(5Z)-5-(carbamoylimino)-3-[(5R)-6,7,8,9-tetrahydro-5H-benzo[7]annulen-5-ylsulfanyl]-2,5-dihydroisothiazole-4-carboxamide 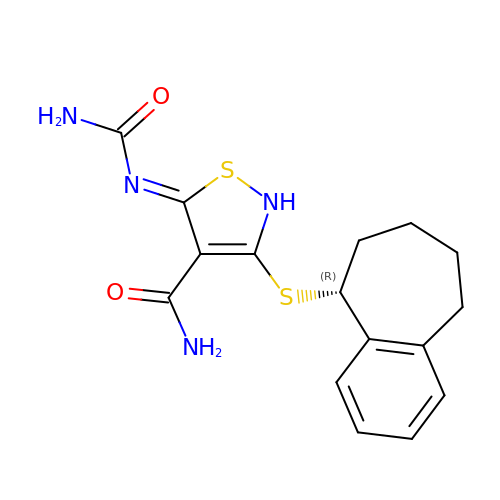| C16 H18 N4 O2 S2 | BLCWVDAFBKECPI-PFMFLNCGSA-N> DMR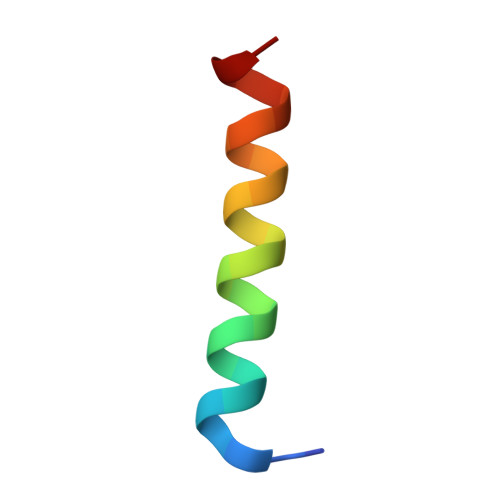PEIRIAQELRRIGDEFNATYAR> MGSDKIHHHHHHMANEATQELFQVLDNTAIILQNELEISYLEAVYETGENLFQKEVLQKEE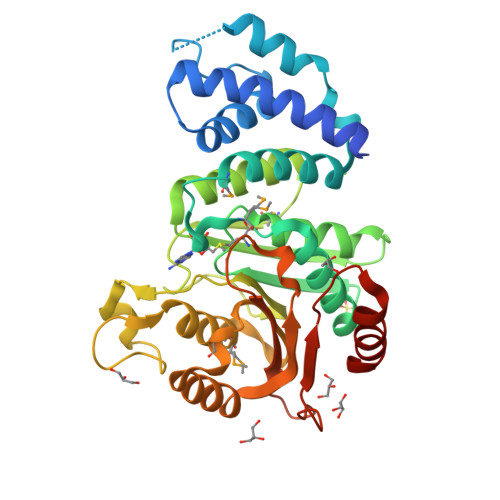LSSEKQLKLQASYESIELENFSNEEIRKGLQLALLKGMKHGIQVNHQMTPDSIGFIVAYLLEKVIQKKKNVSILDPACGTANLLTTVINQLELKGDVDVHASGVDVDDLLISLALVGADLQRQKMTLLHQDGLANLLVDPVDVVISDLPVGYYPDDENAKTFELCREEGHSFAHFLFIEQGMRYTKPGGYLFFLVPDAMFGTSDFAKVDKFIKKNGHIEGIIKLPETLFKSEQARKSILILEKADVDVKPPKEVLLANLSSLTDPSVTAPILAEIENWFKSKQ>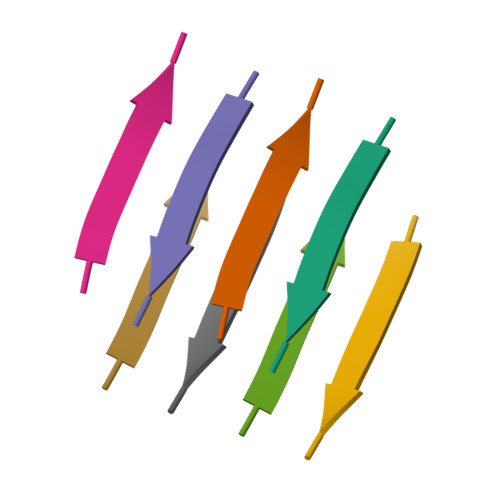[2x]GYMLGS>[4x]MAVPPTYADLGKSARDVFTKGYGFGLIKLDLKTKSENGLEFTSSGSANTETTKVTGSLETKYRWTEYGLTFTEKWNTDNTLGTEITVEDQLARGLKLTFDSSFSPNTGKKNAKIKTGYKREHINLGCDMDFDIA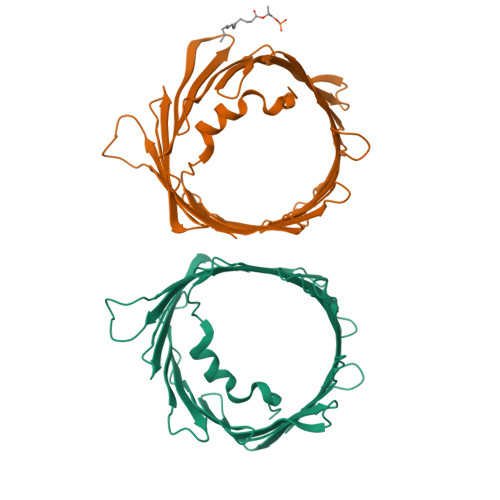GPSIRGALVLGYEGWLAGYQMNFETAKSRVTQSNFAVGYKTDEFQLHTNVNDGTEFGGSIYQKVNKKLETAVNLAWTAGNSNTRFGIAAKYQIDPDACFSAKVNNSSLIGLGYTQTLKPGIKLTLSALLDGKNVNAGGHKLGLGLEFQALEHHHHHH>[3x]APENPGEPGEAGQALFKADFEDGNIGNWRARGTEKLEVVSGIGHNSNRSLKTSSRSETYHGPLVEVLPYLQKGSTVHISFWAMYDEGPATQVINGSLEKEFNRDTANLEYAM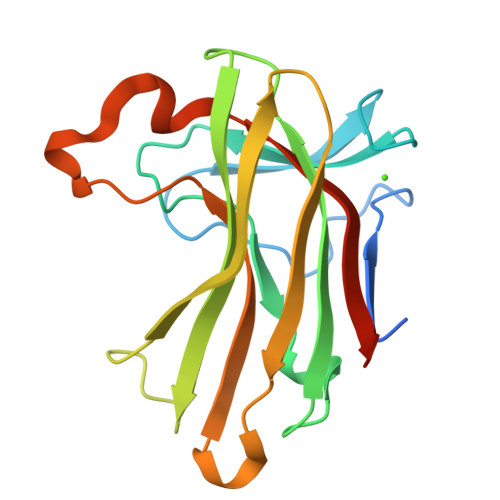FASTTLNKGQWKKIEADIIVPAESTGISGLRMYAETPWKQSSEVTETDTIPFYVDDVQITATEAIAIEK>[2x]GGCCUUAUACAGGGUAGCAUAAUGGGCUAC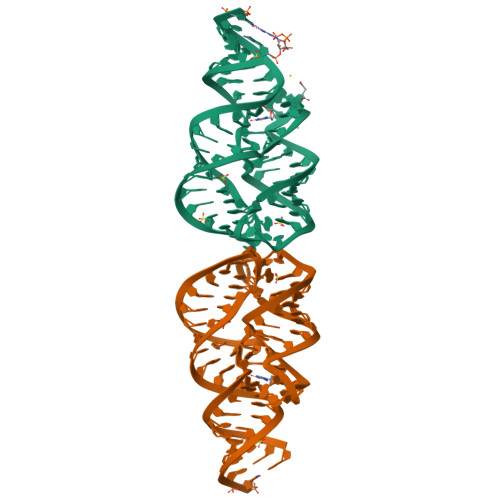UGACCCCGCCUUCAAACCUAUUUGGAGACUAUAAGGUC> MAGAIIENMSTKKLCIVGGILLVFQIIAFLVGGLIAPGPTTAVSYMSVKCVDARKNHHKTKWFVPWGPNHCDKIRDIEEAIPREIEANDIVFSVHIPLPHMEMSPWFQFMLFILQLDIAFKLNNQIRENAEVSMDVSLAYRDDAFAEWTEMAHERVPRKLKCTFTSPKTPEHEGRYYECDVLPFMEIGSVAHKFYLLNIRLPVNEKKKINVGIGEIKDIRLVGIHQNGGFTKVWFAMKTFLTPSIFIIMVWYWRRITMMSR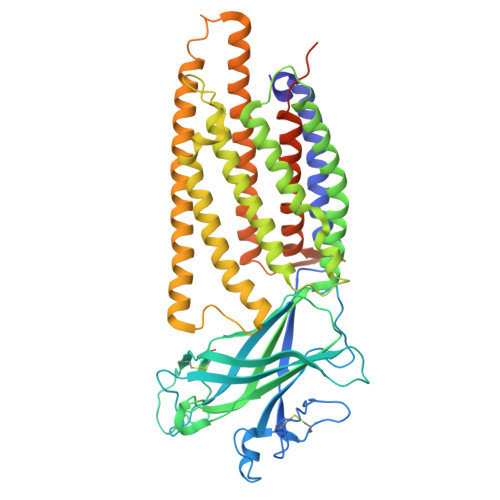PPVLLEKVIFALGISMTFINIPVEWFSIGFDWTWMLLFGDIRQGIFYAMLLSFWIIFCGEHMMDQHERNHIAGYWKQVGPIAVGSFCLFIFDMCERGVQLTNPFYSIWTTDIGTELAMAFIIVAGICLCLYFLFLCFMVFQVFRNISGKQSSLPAMSKVRRLHYEGLIFRFKFLMLITLACAAMTVIFFIVSQVTEGHWKWGGVTVQVNSAFFTGIYGMWNLYVFALMFLYAPSHKNYGEDQSNGDLGVHSGEELQLTTTITHVDGPTEIYKLTRKEAQE> AVKRPAATK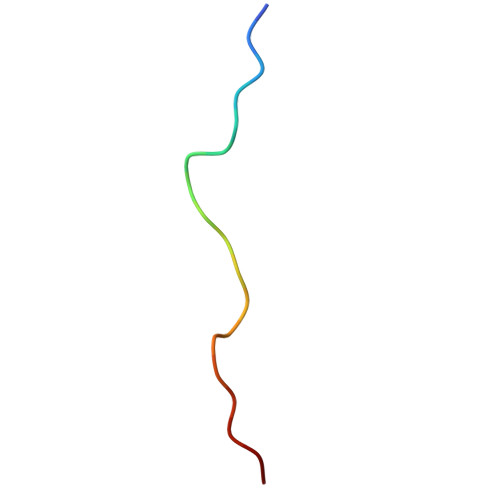KAGQAKKKKL> MHHHHHHSSGRENLYFQGNFDYMFKLLIIGNSSVGKTSFLFRYADDTFTPAFVSTVGIDFKVKTVYRHEKRVKLQIWDTAGQE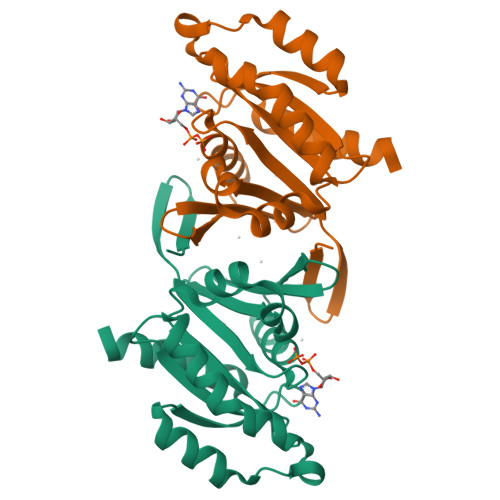RYRTITTAYYRGAMGFILMYDITNEESFNAVQDWATQIKTYSWDNAQVILVGNKCDMEEERVVPTEKGQLLAEQLGFDFFEASAKENISVRQAFERLVDAICDKMSDS> EMPQIETRVILVQ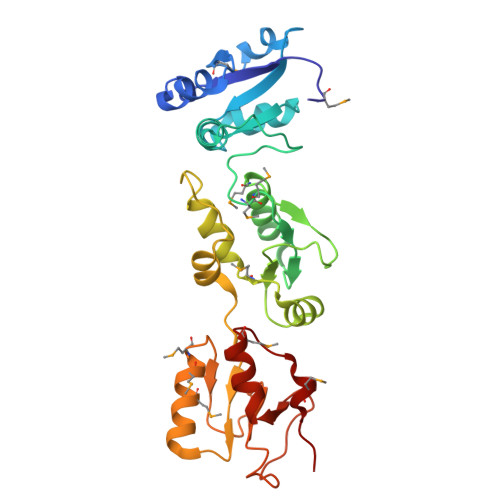EAGKQEELIKALKDIKVGFVKMESVEEFEGLDSPEFENVFVVTDFQDSVFNDLYKADCRVIGPPVVLNCSQKGEPLPFSCRPLYCTSMMNLVLCFTGFRKKEELVRLVTLVHHMGGVIRKDFNSKVTHLVANCTQGEKFRVAVSLGTPIMKPEWIYKAWERRNEQDFYAAVDDFRNEFKVPPFQDCILSFLGFSDEEKTNMEEMTEMQGGKYLPLGDERCTHLVVEENIVKDLPFEPSKKLYVVKQEWFWGSIQMDARAGETMYLYEK> SDQTWVQCDACLKWRKLPDGMDQLPEKWYCSNNPDPQFRNCEVPEEPEDE;> ARTKQTARK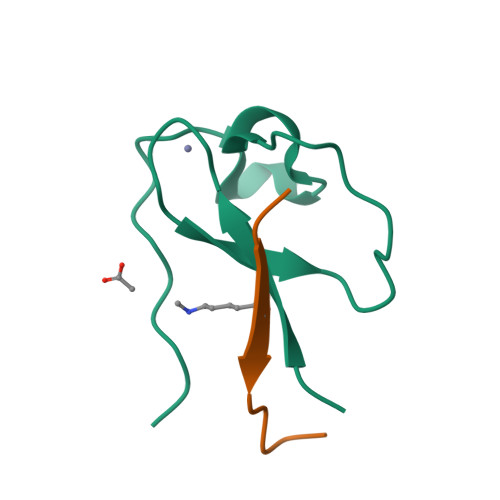ST> MTATQGKCPVMHGGATTVNISTAEWWPKALNLDILSQHDRKTNPMGPDFNYQEEVQKLDAALKQDLQALMTDSQDWWPADWGHYGGLMIRLTWHAAGTYRIADGRGGAGTGNQRFAPLNSWPDNTNLDKARRLLWPIKQKYGNKLSWADLIAYAGTIAYESMGLKTFGFAFGREDIWHPEKDIYWGPEKEWFPPSTNPNSRYTGDRELENPLAAVTMGLIYVNPEGVDGNPDPLKTAHDVRVTFARMAMNDEETVALTAGGHTVGKCHGNGNAALLGPEPEGADVEDQGLGWINKTQSGIGRNAVTSGLEGAWTPHPTQWDNGYFAVCSLNYDWELKKNPAGAWQWEPINPREEDLPVDVEDPSIRRNLVMTD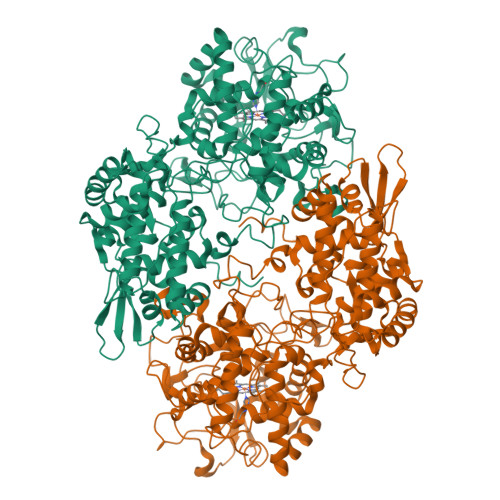ADMAMKMDPEYRKISERFYQDPAYFADVFARAWFKLTHRDMGPKARYIGPDVPQEDLIWQDPIPAGNRNYDVQAVKDRIAASGLSISELVSTAWDSARTYRNSDKRGGANGARIRLAPQKDWEGNEPDRLPKVLAVLEGISAATGATVADVIVLAGNVGVEQKARAAGVEIVLPFAPGRGDATAEQTDTESFAVLEPIHDAIATGSSRTMRQRLKNCCLIATQLLGLTAPEMTVLIGGLRVLGTNHGGTKHVVFTDREGVLTNDFFVNLTDMNYLWKPAGKNLYEICDRKTNQVKWTATRVDLVFGSNSILRAYSELYAQDDNKEKFVRDFVAAWTKVMNADRFDLD> HHHHHHMQHLVLIGFMGSGKSSLAQELGLALKLEVLDTDMIISERVGLSVREIFE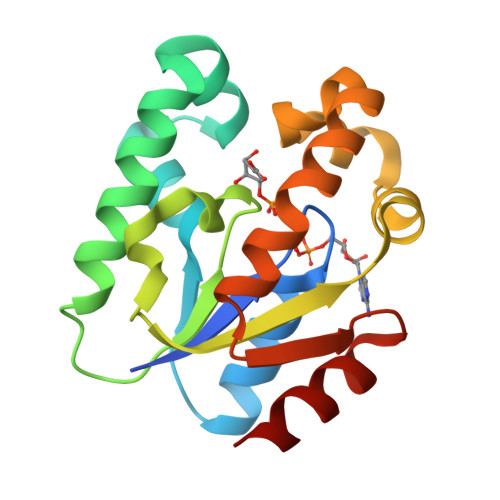ELGEDNFRMFEKNLIDELKTLKTPHVISTGGGIVMHENLKGLGTTFYLKMDFETLIKRLNQKEREKRPLLNNLTQAKELFEKRQALYEKNASFIIDARGGLNNSLKQVLQFIA>[4x]MALDEAPAEARPGSRAVELEIDGRSRIFDIDDPDLPKWIDEEAFRSDDYPYKKKLDREEYEETLTKLQIELVKVQFWMQATGKRVMAVFEGRDAAGKGGAIHATTANMNPRSARVVALTKPTETERGQWYFQRYVATFPTAG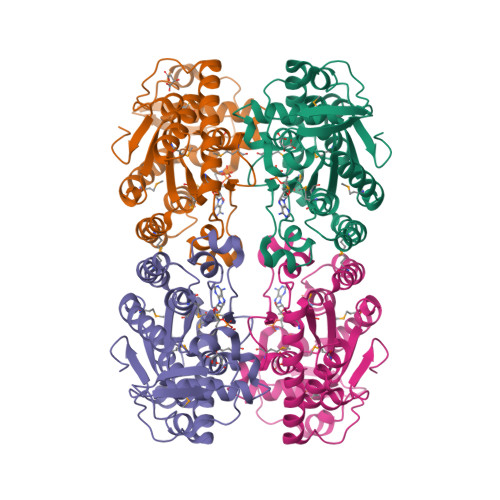EFVLFDRSWYNRAGVEPVMGFCTPDQYEQFLKEAPRFEEMIANEGIHLFKFWINIGREMQLKRFHDRRHDPLKIWKLSPMDIAALSKWDDYTGKRDRMLKETHTEHGPWAVIRGNDKRRSRINVIRHMLTKLDYDGKDEAAIGEVDEKILGSGPGFLR ABC toxins are secreted endotoxins produced by bacterial pathogens of insects and animals. Originally described as Tcs (for toxin complexes), and more recently described as A5BC toxins in reference to their stoichiometry, all three subunits (A, B and C) are required to assemble a complex with full toxicity. YenTcA is the pore-forming and membrane-binding module of YenTc. It has an unusual architecture amongst ABC toxins, in that it is encoded by four genes, two of which represent an apparently split tcA-like gene (yenA1 and yenA2) and two of which encode functional endochitinases (chi1 and chi2).

The current manuscript reports a substantially improved structure of YenTcA isolated from a transposon mutant of the native Y. entomophaga, in its soluble (pre-pore) conformation, determined by single-particle cryo-EM and 3D reconstruction. The resolution of the structure, estimated at 4.4 Å, allows unequivocal assignment of all four unique polypeptide chains within the structure, with an overall atomic model able to be built that accounts for 75% of the complete amino acid sequence. YenTcA is assembled from five symmetrically-arranged protomers, each comprising a single copy of YenA1, YenA2, Chi2 and Chi1. Each protomer contributes a pair of extended α-helices that form a funnel-shaped longitudinal pore at the core of the complex that widens into a β-sandwich domain (the TcB-binding domain) at one end and is enclosed at the opposite end by a ring of five neuraminidase-like domains (again, one is contributed by each protomer). This structure—the pore-forming apparatus—is entirely encoded by the YenA2 chain. A predominantly α-helical shell incorporating regions of both YenA1 and YenA2 forms the next layer, encapsulating the longitudinal pore. The Chi2 proteins form an equatorial ring around the lower half of the α-helical shell, while five, leg-like protrusions emerge from the base of the complex. The molecular interface between YenA1 and YenA2 within a single protomer represents a buried surface area of 2709 Å2 and the C-terminus of YenA1 is in close proximity to the N-terminus of YenA2 (separated by approximately 16 Å). Most notably, a ring of five histidines (H996) forms a constriction (to ~6 Å diameter) about 20 Å above the tip, while the final closure involves hydrophobic interactions of the sidechains of the five L990 residues. Chi2 is incorporated into the overall structure such that its substrate cleft is solvent exposed and opens approximately downwards.

>MDKYNNYSNVIKNKSSISPLLAAAAKIEPEITVLSSASKSNRSQYSQSLADTLLGLGYRSIFDIAKVSRQRFIKRHDESLLGNGAVIFDKAVSMANQVLQKYRKNRLEKSNSPLVPQTSSSTDASSESQTNKLPEYNQLFPEPWDNFCRPGAIEALDSPASYLLDLYKFIQSVELDGSNQARKLETRRADIPKLSLDNDALYKEVTALSIVNDVLSGSAREYIDQSGQADKAVNQILGDTHFPFTLPYSLPTQQINKGLGASNIELGTVIQRVDPQFSWNTTQEKYNQVLLAYTQLSSEQIALLSLPDVFTQNFLTQTELSAGYLSASTTEILAEKDLSRHGYIVKAADNIKGPTQLVEHSDASYDVIELTCTNQAKETITVKLRGENIITYQRTKARMVPFDNSSPFSRQLKLTFVAEDNPSLGNLDKGPYFANMDIYAAEWVRENVSSETMVSRPFLTMTYRIAIAKAGASLEELQPEADAFFINNFGLSAEDSSQLVKLVAFGDQTGSKAEEIESLLSCGENLPIVSPNVIFANPIFGSYFNDEPFPAPYHFGGVYINAHQRNAMTIIRAEGGREIQSLSNFRLERLNRFIRLQRWLDLPSHQLDLLLTSVMQADADNSQQEITEPVLKSLGLFRHLNLQYKITPEIFSSWLYQLTPFAVSGEIAFFDRIFNREQLFDQPFILDGGSFTYLDAKGSDAKSVKQLCAGLNISAVTFQFIAPLVQSALGLEAGTLVRSFEVVSSLYRLVSIPQTFGLSTEDGLILMNILTDEMGYLAKQPAFDDKQTQDKDFLSIILKMEALSAWLTKNNLTPASLALLLGVTRLAVVPTNNMVTFFKGIANGLSENVCLTTDDFQRQELEGADWWTLLSTNQVIDDMGLVLDIHPVWGKSDEEMLMEKIQSIGVSNDNNTLSIIVQILIQAKNAQENLLSQTISAEYGVERSVVPLQLRWLGSNVYSVLNQVLNNTPTDISSIVPKLSELTYSLLIYTQLINSLKLNKEFIFLRLTQPNWLGLTQPKLSTQLSLPEIYLITCYQDWVVNANKNEDSIHEYLEFANIKKTEAEKTLVDNSEKCAELLAEILAWDAGEILKAASLLGLNPPQATNVFEIDWIRRLQTLSEKTMISTEYLWQMGDLTENSEFSLKEGVGEAVMAALKAQGDSDNV[5x];>MSNSIEAKLQEDLRDALVDYYLGQIVPNSKDFTNLRSTIKNVDDLYDHLLLDTQVSAKVITSRLSLVTQSVQQYINRIALNLEPGLSINQQEATDWEEFANRYGYWAANQQLRMFPEIYVDPTLRLTKTEFFFQLESALNQGKLTDDVAQKAVLGYLNNFEEVSNLEIIAGYQDGIDIENDKTYFVARTRMQPYRYFWRSLDASQRNANSQELYPTAWSEWKAISVPLENVANGIVRPIMMDNRLYISWFEVAEEKETDSDGNIIVSGRYRTKIRLAHLGFDGVWSSGTTLREEVLADQMEEMIAVVDRMEDEPRLALVAFKEMSESWDVVFSYICDSMLIESSNLPTTTHPPKPGDGDKGLSDLDDYGANLVWFYLHETANGGKAEYKQLILYPVIINRDWPIELDKTHQGDFGTVDDFTLNSNYTGDELSLYLQSSSTYKYDFSKSKNIIYGIWKEDANNNRCWLNYKLLTPEDYEPQINATLVMCDKGDVNIITGFSLPNGGVDAGGKIKVTLRVGKKLRDKFQIKQFSQTQYLQFPEASSADVWYIGKQIRLNTLFAKELIGKASRSLDLVLSWETQNSRLEEAILGGAAELIDLDGANGIYFWELFFHMPFMVSWRFNVEQRYEDANRWVKYLFNPFECEDEPALLLGKPPYWNSRPLVDEPFKGYSLTQPSDPDAIAASDPIHYRKAVFNFLTKNIIDQGDMEYRKLQPSARTLARLSYSTASSLLGRRPDVQLTSFWQPLTLEDASYKTDSEIRAIEMQSQPLTFEPVVHDQTMSAVDNDIFMYPMNNELRGLWDRIENRIYNLRHNLTLDGKEINMDLYDSSISPRGLMKQRYQRVVTARNASKMNFKVPNYRFEPMLNRSKSGVETLIQFGSTLLSLLERKDSLSFDAYQMIQSGDLYRFSIDLQQQDIDINKASLEALQVSKQSAQDRYDHFKELYDENISSTEQKVIELQSQAANSLLMAQGMRTAAAALDVIPNIYGLAVGGSHWGAPLNAAAEIIMIKYQADSSKSESLSVSESYRRRRQEWELQYKQAEWEVNSVEQQINLQNMQIKAANKRLEQVEAQQQQAMALLDYFSERFTNESLYTWLISQLSSLYLQAYDAVLSLCLSAEASLLYELNLGEQSFVGGGGWNDLYQGLMAGETLKLALMRMERVYVEQNSRRQEITKTISLKALLGESWPAELNKLKQKTPINFNLEEQIFVEDYQELYQRRIKSVSVSLPMLVGPYEDVCAQLTQTSSSYSTRADLKTVENMLTKRTFADTPHLVRSIQPNQQISLSTGVNDSGLFMLNFDDERFLPFEGSGVDSSWRLQFTNLKQNLDSLNDVILHVKYTAAIGSSTFSQGVRKILANINNDE[5x];>[5x]MVNKYTYTSSKAMSDISDVIGEPLAAWDSQVGGRVFNVIFDGKVYTNTYWVERWQVPGIGSSDGNPHNAWKFVRAATADEINKIGNPTTADVKPTENIPSPILVEDKYTEETYSRPDVNFKEDGSQGNLSYTATRVCAPMYNHYVGDKTKPKLSAYITDWCQYDARLDGGGSKEEERGRGFDLATLMQNPATYDRLIFSFLGICGDIGNKSKKVQEVWDGWNAQAPSLGLPQIGKGHIVPLDPYGDLGTARNVGLPPESADTSIESGTFLPYYQQNRAAGLLGGLRELQKKAHAMGHKLDLAFSIGGWSLSSYFSALAENPDERRVFVASVVDFFVRFPMFSCVDIDWEYPGGGGDEGNISSDKDGENYVLLIKELRSALDSRFGYSNRKEISIACSGVKAKLKKSNIDQLVANGLDNIYLMSYDFFGTIWADYIGHHTNLYSPKDPGEQELFDLSAEAAIDYLHNELGIPMEKIHLGYANYGRSAVGGDLTTRQYTKNGPALGTMENGAPEFFDIVKNYMDAEHSLSMGKNGFVLMTDTNADADFLFSEAKGHFISLDTPRTVKQKGEYAAKNKLGGVFSWSGDQDCGLLANAAREGLGYVADSNQETIDMGPLYNPGKEIYLKSISEIKSK> GMLFESINTGCLDGNDTPWMPFAPYSNDVMVKYFKIDPVRGETITLLKAPAGMEMPRHHHTG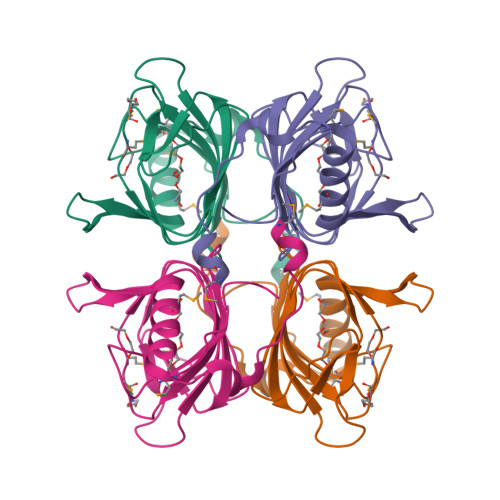TVIVYTVQGSWRYKEHDWVAHAGSVVYETASTRHTPQSAYAEGPDIITFNIVAGELLYLDDKDNIIAVENWKTSMDRYLNYCKAHGIRPKDLSTFEG> MVNVKVEFLGGLDAIFGKQRVHKIKMDKEDPVTVGDLIDHIVSTMINNPN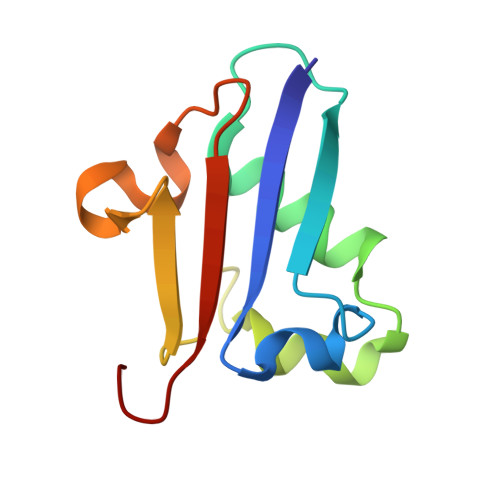DVSIFIEDDSIRPGIITLINDTDWELEGEKDYILEDGDIISFTSTLHGG> MKRAVITGLGIVSSIGNNQQEVLASLREGRSGITFSQELKDSGMRSHVWGNVKLDTTGLIDRKVVRFMSDASIYAFLSMEQAIADAGLSPEAYQNNPRVGLIAGSGGGSPRFQVFGADAMRGPRGLKAVGPYVVTKAMASGVSACLATPFKIHGVNYSISSACATSAHCIGNAVEQIQLGKQDIVFAGGGEELCWEMACEFDAMGALSTKYNDTPEKASRTYDAHRDGFV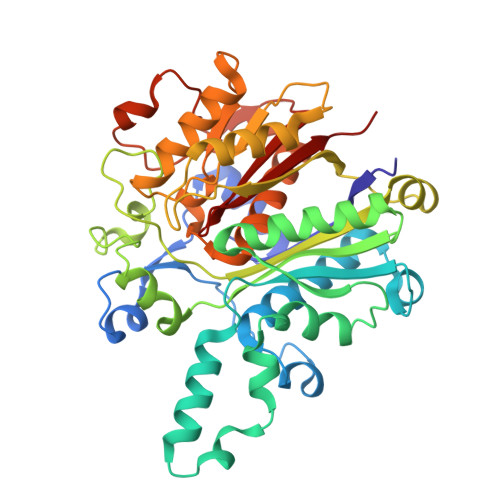IAGGGGMVVVEELEHALARGAHIYAEIVGYGATSDGADMVAPSGEGAVRCMKMAMHGVDTPIDYLNSHGTSTPVGDVKELAAIREVFGDKSPAISATKAMTGHSLGAAGVQEAIYSLLMLEHGFIAPSINIEELDEQAAGLNIVTETTDRELTTVMSNSFGFGGTNATLVMRKLK> MAVPFVEDWDLVQTLGEGAYGEVQLAVNRVTEEAVAVKIVDMKRAVDCPENIKKEICINKMLNHENVVKFYGHRREGNIQYLFLEYCSGGELFDRIEPDIGMPEPDAQRFFHQLMAGVVYLHGIGITHRDIKPENLLLDERDNLKISDFGLATVFRYNNRERLLNKMCGTLPYVAPELLKRREFHAEPVDVWSCGIVLTAMLAGELPWDQPSDSCQEYSDWKEKKTYLNPWKKIDSAPLALLHKILVENPSARITIPDIKKDRWYNKPLK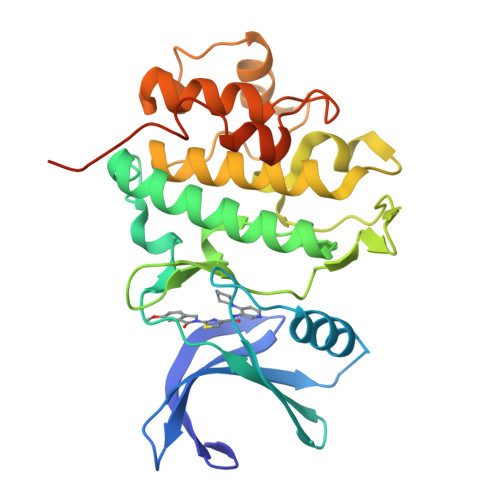KGAKRPRVTSGGVSESPSG> MGAQVLRGTVTDFPGFDERADAETLRKAMKGLGTDEESILTLLTSR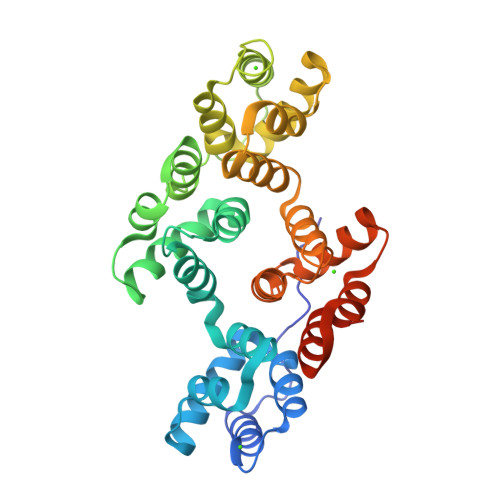SNAQRQEISAAFKTLFGRDLLDDLKSELTGKFEKLIVALMKPSRLYDAYELKHALKGAGTNEKVLTEIIASRTPEELRAIKQVYEEEYGSSLEDDVVGDTSGYYQRMLVVLLQANRDPDAGIDEAQVEQDAQALFQAGELKWGTDEEKFITIFGTRSVSHLRKVFDKYMTISGFQIEETIDRETSGNLEQLLLAVVKSIRSIPAYLAETLYYAMKGAGTDDHTLIRVMVSRSEIDLFNIRKEFRKNFATSLYSMIKGDTSGDYKKALLLLCGEDDHHHHHHHHHH METHYL 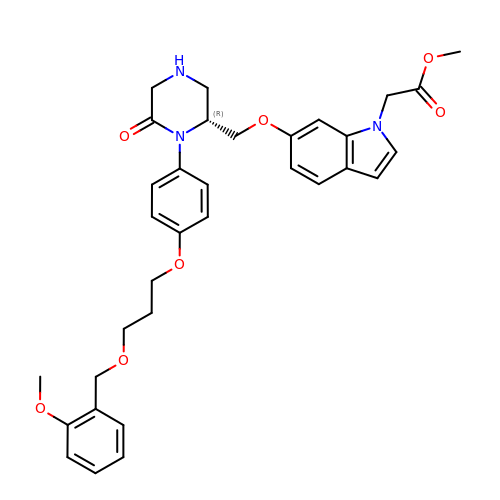(6-{[(2R)-1-(4-{3-[(2-METHOXYBENZYL)OXY]PROPOXY}PHENYL)-6-OXOPIPERAZIN-2-YL]METHOXY}-1H-INDOL-1-YL)ACETATE | C33 H37 N3 O7 | KWJWTGNGIVRJJK-HHHXNRCGSA-N> DVLNVSGHRLGTAEIESALVAHPKIAEAAVVGIPHAIKGQAIYAYVTLNCGEEPSPELYAEVRNWVRKEIGPLATPDVLHWTDSLPKTRSGKIMRRILRKIAAGDTSNLGDTSTLAD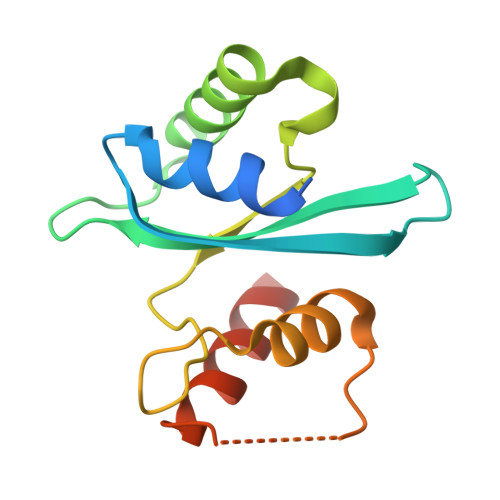PGVVEKLLEEKQAIAMPS ethyl 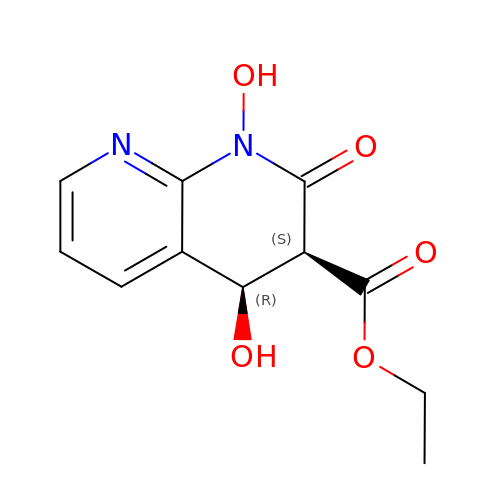1,4-dihydroxy-2-oxo-1,2-dihydro-1,8-naphthyridine-3-carboxylate | C11 H12 N2 O5 | MTVPGFFXVTZGIM-YUMQZZPRSA-N> NKGA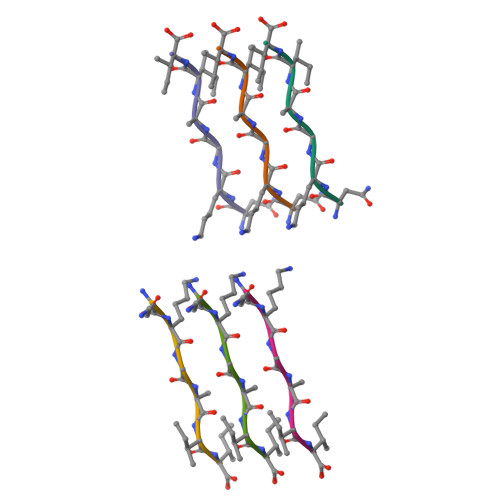II>[2x]MGSSHHHHHHSQDPNSASPAMVPLRQLFVDGEWRPPAQGRRLPVVNPTTEAHIGEIPAGTAEDVDAAVAAARAALKRNRGRDWARAPGAVRAKYLRAIAAKVIERKPELAKLEALDCGKPYDEAAWDMDDVAGCFEYFADQAEALDKRQNSPVSLPMETFKCHLRREPIGVVGLITPWNYPLLMATWKIAPALAAGCTAVLKPSELASVTCLELADICKEVGLPSGVLNIVTGLGPDAGAPLSAHPDVDKVAFTGSFETGKKIMASAAPMVKPVTLELGGKSPIVVFDDVDIDKAVEWTLFGCFWTNGQICSATSRLLIHTKIAKKFNERMVAWAKNIKVSDPLEEGCRLGPVVSEGQYEKIKKFISNAKSQGATILTGGVRPAHLEKGFFIEPTIITDITTSMEIWREEVFGPVLCVKEFSTEDEAIELANDTQYGLAGAVISGDRERCQRLSEEIDAGCIWVNCSQPCFCQAPWGGN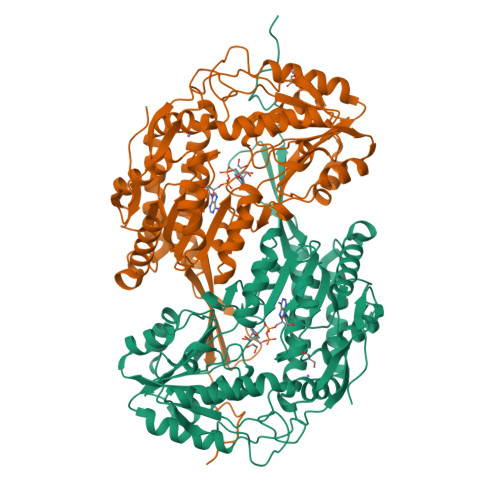KRSGFGRELGEGGIDNYLSVKQVTEYISDEPWGWYQSPSKL> LAPRKQLATK;> GPLGSPEFMAQGTLIRVTPEQPTHAVCVLGTLTQLDICSSAPEDCTSFSINASPGVVVDIAHSPPAKKKSTGSSTWPLDPGVEVTLTMKAASGSTGDQKVQISYYGPKTPPVKALLYLTAVEISLCADITRTGKVKPTRAVKDQRTWTWGPCGQGAILLVNCDRDNLESSAMDCEDDEVLDSEDLQDMSLMTLSTKTPKDFFTNHTLVLHVARSEMDKVRVFQATRGKLSSKCSVVLGPKWPSHYLMVPGGKHNMDFYVEALAFPDTDFPGLITLTISLLDTSNLELPEAVVFQDSVVFRVAPWIMTPNTQPPQEVYACSIFENEDFLKSVTTLAMKAKCKLTICPEEENMDDQWMQDEMEIGYIQAPHKTLPVVFDSPRNRGLKEFPIKRVMGPDFGYVTRGPQTGGISGLDSFGNLEVSPPVTVRGKEYPLGRILFGDSCYPSNDSRQMHQALQDFLSAQQVQAPVKLYSDWLSVGHVDEFLSFVPAPDRKGFRLLLASPRSCYKLFQEQQNEGHGEALLFEGIKKKKQQ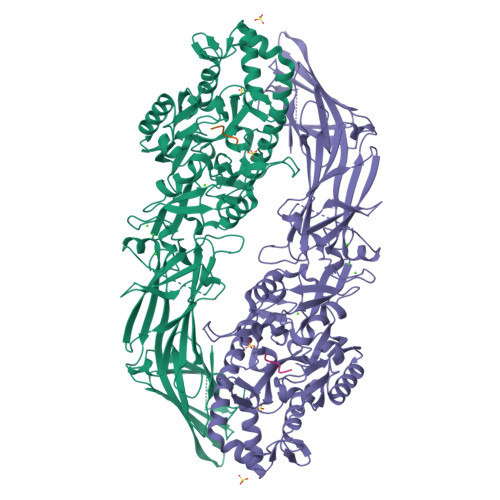KIKNILSNKTLREHNSFVERCIDWNRELLKRELGLAESDIIDIPQLFKLKEFSKAEAFFPNMVNMLVLGKHLGIPKPFGPVINGRCCLEEKVCSLLEPLGLQCTFINDFFTYHIRHGEVHAGTNVRRKPFSFKWWNMVP> YPHPAYPMPFITTILGGLYPSKSILLSGTVLPSAQRFHINLCSGNHIAFHLNPRF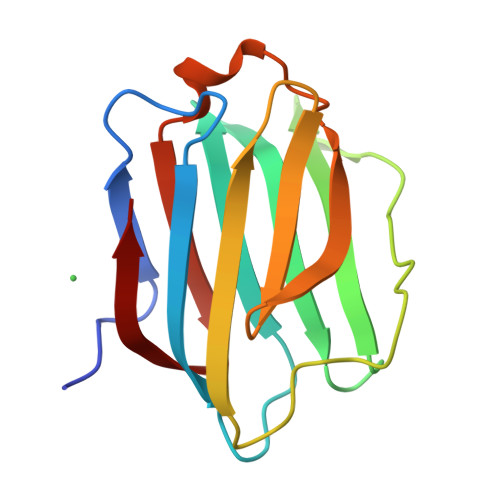DENAVVRNTQIDNSWGSEERSLPRKMPFVRGQSFSVWILCEAHCLKVAVDGQHLFEYYHRLRNLPTINRLEVGGDIQLTHVQT> FRSCEVPTRLNSASLKQPYITQNYFPVGTVVE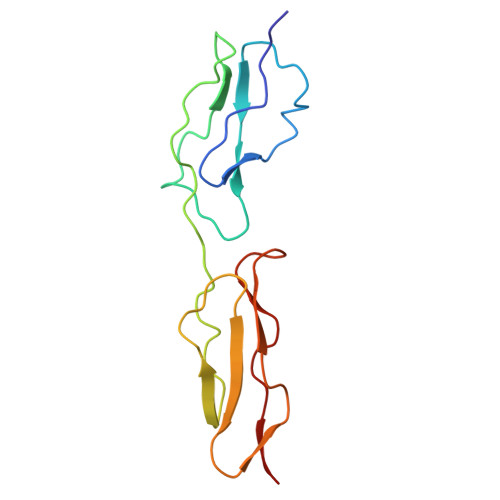YECRPGYRREPSLSPKLTCLQNLKWSTAVEFCKKKSCPNPGEIRNGQIDVPGGILFGATISFSCNTGYKLFGSTSSFCLISGSSVQWSDPLPECREH>[4x]GPLGSRPFRFSPEPTLEDIRRLHAEFAAERDWEQF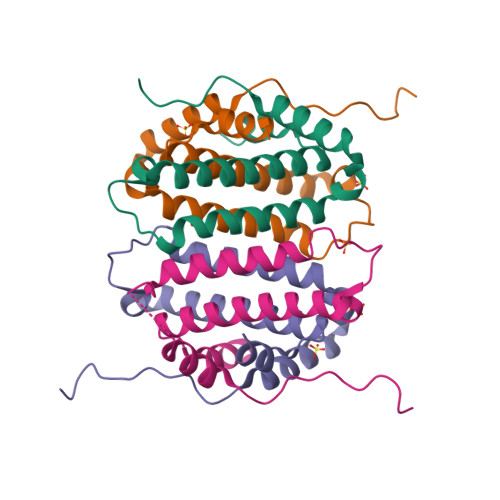HQPRNLLLALVGEVGELAELFQWKSDTEPGPQAWPPKERAALQEELSDVLIYLVALAARCHVDLPQAVISKMDTNR>[2x]ITLLTLIKTAEHWARQDIRTIEDSKLRALLTLCAVMTRKFSKSQLSLLCETHLRREGLG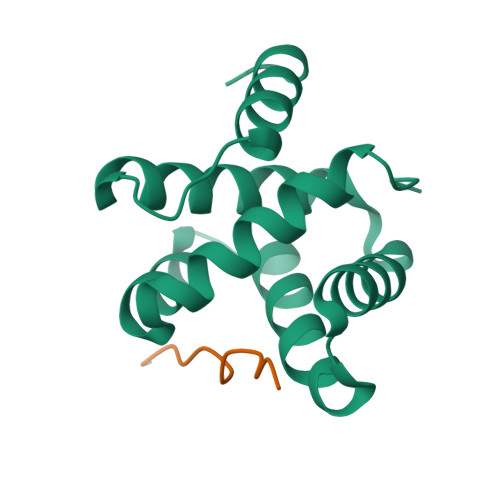QDQAEPVLEVYQRLHSDKGGSFEAALWQQWDRQSLIMFITAFLNIALQLPCES;>[2x]TPTVAPPAPVYR>RSYEQMETDGERQNATEIRASVGKMIDGIGRFYIQMCTELKLSDYEGRLIQNSLTIERMVLSAFDERRNKYLEEHPSAGKDPKKTGGPIYRRVDGKWRRELILYDKEEIRRIWRQANNGDDATAGLTHMMIWHSNLNDATYQRTRALVRTGMDPRMCSLMQGSTLPRRSGAAGAAVKGVGTMVMELIRMIKRGINDRNFWRGENGRRTRIAYERMCNILKGKFQTAAQRTMVDQVRESRNPGNAEFEDLIFLARSALILRGSVAHKSCLPACVYGSAVASGYDFEREGYSLVGIDPFRLLQNSQVYSLIRPNENPAHKSQLVWMACHSAAFEDLRVSSFIRGTKVVPRGKLSTRGVQIASNENMETMESSTLELRSRYWAIRTRSGGNTNQQRASSGQISIQPTFSVQRNLPFDRPTIMAAFTGNTEGRTSDMRTEIIRLMESARPEDVSFQGRGVFELSDEK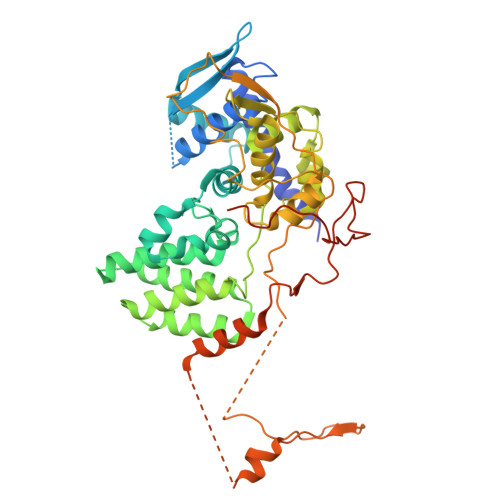ATSPIVPSFDMSNEGSYFFGDNAEEYDNLEHHHHHH[9x]>[12x]MIVRTQNSESKIKEFFEFCKENEVEFVDFRFSDIKGTWNHIAYSFGALTHGMLKEGIPFDASCFKGWQGIEHSDMILTPDLVRYFIDPFSADVSVVVFCDVYDVYKNQPYEKCPRSIAKKALQHLKDSGLGDVAYFGAENEFFIFDSIKIKDASNSQYYEVDSEEGEWNRDRSFENGVNFGHRPGKQGGYMPVPPTDTMMDIRTEIVKVLNQVGLETFVVHHEVAQAQGEVGVKFGDLVEAADNVQKLKYVVKMVAHLNGKTATFMPKPLYGDNGSGMHTHVSVWKNNENLFSGETYKGLSEFALHFLGGVLRHARGLAAFTNASTNSYKRLIPGYEAPSILTYSANNRSASVRIPYGISKNSARFEFRFPDSSSNPYLAFAAILMAGMDGVKNKIDPGEAMDINLFKLTLDEIREKGIKQMPHTLRRSLEEMLADKQYLKESQVFSEEFIQAYQSLKFNAEVFPWESKPHPFEFITTYSC

The GS in H. pylori (Hpy GS) is a critical enzyme that is involved in processing the ammonia released by urease activity, and nitrogen metabolism. GS is an enzyme involved in the biosynthetic reaction producing glutamine from the condensation of glutamate and ammonia. This enzyme is present in all living organisms and is a large homo-oligomeric complex composed of eight, ten, or twelve subunits assembled into two face-to-face rings. Although the structural and sequence information of Hpy GS indicate its relationship with GS I-β due to the presence of a specific 25-amino acid residues (residues 155–179), the adenylation site (NLYDLP) found in similar homologs is replaced in Hpy GS (NLF407KLT), suggesting a lack of the adenylation regulatory mechanism in Hpy GS.

The substrate-bound form of Hpy GS (Hpy GSsub) was obtained in the presence of ATP and PPT, which is a structural analogue of glutamate. Hpy GSsub was determined at 2.9 Å and refined to crystallographic Rwork and Rfree values of 16.45% and 24.27%, respectively. In Hpy GSsub, twelve subunits in the asymmetric unit were also highly similar with r.m.s.d. values of 0.29–0.36 Å for 475 Cα atoms in residues 7–481. However, although ATP and PPT were added to Hpy GS, ATP/ADP substrates were clearly identified in all subunits, whereas PPT/P3P substrates were not identified in most of the subunits of Hpy GS. Among twelve subunits, PPT was not phosphorylated, resulting in a substrate-bound form with PPT and ATP in three subunits. In only one subunit, PPT was phosphorylated by ATP hydrolysis, resulting in an intermediate state with P3P and ADP. PPT was bound by six hydrogen bonds with Hpy GS (NP to E141 Oε1/G275 O, OTP to R331 Nε, OP to H279 Nε2/R331 NH2, and OεB to R369 NH2), and P3P was bound by seven hydrogen bonds, where the O13 atom additionally formed a hydrogen bond with R349 NH2. The possible ammonium binding site was blocked by the methyl group of P3P, acting as an inhibitor. In both the Hpy GSint and Hpy GSsub structures, one magnesium ion was identified in the n1 metal binding site. The side chain of E337 in the Hpy GSapo structure was disordered, demonstrating the flexibility of the Glu flap, whereas the side chain of E337 in the Hpy GSsub structure formed strong hydrogen bonds with the N274 Oδ1 and D60 Nδ2 of the adjacent subunit.ethyl 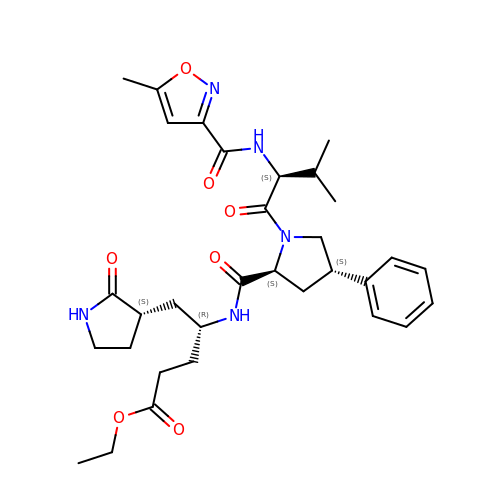(4R)-4-[[(2S,4S)-1-[(2S)-3-methyl-2-[(5-methyl-1,2-oxazol-3-yl)carbonylamino]butanoyl]-4-phenyl-pyrrolidin-2-yl]carbonylamino]-5-[(3S)-2-oxidanylidenepyrrolidin-3-yl]pentanoate | C32 H43 N5 O7 | VXYKULSXGSKGQQ-OSKYGDQXSA-N> SNAMTNSSEKQWERIQQLEKEHVEVYRELLITLDRLYLIRKHNHAVILSHTQQRLLEIRHQLQINLEKTALLIRLLEKPDNTNVLFTKLQNLLEESNSLDYELLQSLGAQSSLHKQLIESRAERDELMSKLIELSSKFPKPTIPPDDSDTAGKQVEVEKENETIQELMIALQIHSGYTNISYTI;> SNAMSLILDDIILSLTNANERTPPQALKTTLSLLYEKSKQYGLSSPQLQALVRLLCETSIIDTVTKVYIVENCFLPDGYLTKELLLEIINHLGTPTVFSRYRIQTPPVLQSALCKWLVHVYFLFPVHSEREHNISSSIWLHLWQFSFLQKWITPLVIWQATTPVDVKPWKLSIIKRCAMHPGYRDAPGSATLILQRFQCLVGASSQITESIITINCNRKTLKSHRNLKLDAHFLSILKRILSRAHPANFPADTVQNTIDMYLSEIHQLGADSIYPLRLQSLPEYVPSDSTVSLWDVTSLEQLAQNWPQLHIPNDVDYMMKPSLNSNVLLPRKVMSRDSLKHLYSSIILIKNSRDESSSPYEWCIWQLKRCFAHQIETPQEVIPIIISVSSMDNKLSSRIIQTFCNLKYLKLDELTLKKVCGGILPLWKPELISGTREFFVKFMASIFMWSTRDGHDNNCTFSETCFYVLQMITNWVLDDKLIALGLTLLHDMQSLLTLDKIFNNATSNRFSTMAFISSLDILTQLSKQTKSDYAIQYLIVGPDIMNKVFSSDDPLLLSAACRYLVATKNKLMQYPSTNKFVRMQNQYIMDLTNYLYRNKVLSSKSLFGVSPDFFKQILENLYIPTADFKNAKFFTITGIPALSYICIIILRRLETAENTKIKFTSGIINEETFNNFFRVHHDEIGQHGWIKGVNNIHDLRVKILMHLSNTANPYRDIAAFLFTYLKSLSKYSVQNS;> SNAMDVEKDVLDVYIKNLENQIGNKRYFLKQAQGAIDEITKRSLDTEGKPVNSEVFTELLRKPMFFSERADPIGFSLTSNFLSLRAQSSSEWLSLMNDQSVDQKAMLLLQNNINSDLKELLRKLQHQMTIMDSKKQDHAHIRTRKARNKELWDSLADFLKGYLVPNLDDNDESIDSLTNEVMLLMKRLIEHDLNLTLNDFSSKTIPIYRLLLRANIITVIEGSTNPGTKYIKLIDFNETSLT;> MSTPRKAAGNNENTEVSEIRTPFRERALEEQRLKDEVLIRNTPGYRKLLSASTKSHDILNKDPNEVRSFLQDLSQVLARKSQGNDTTTNKTQARNLIDELAYEESQPEENELLRSRSEKLTDNNIGNETQPDYTSLSQTVFAKLQERDKGLKSRKIDPIIIQDVPTTGHEDELTVHSPDKANSISMEVLRTSPSIGMDQVDEPPVRDPVPISITQQEEPLSEDLPSDDKEETEEAENEDYSFENTSDENLDDIGNDPIRLNVPAVRRSSIKPLQIMDLKHLTRQFLNENRIILPKQTWSTIQEESLNIMDFLKQKIGTLQKQELVDSFIDMGIINNVDDMFELAHELLPLELQSRIESYLF;> SNAMDTEALANYLLRQLSLDAEENKLEDLLQRQNEDQESSQEYNKKLLLACGFQAILRKILLDARTRATAEGL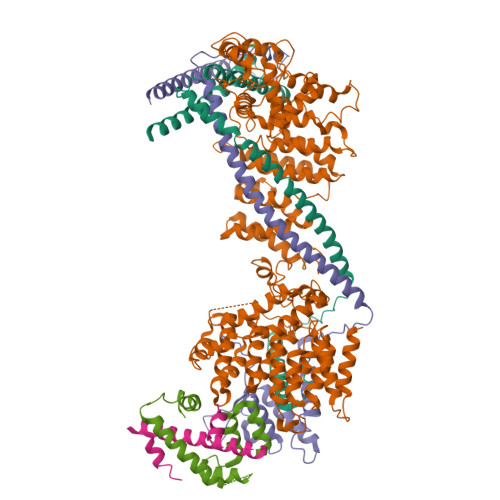REVYPYHIEAATQAFLDSQ> STSHCRFYENKYPEIDDIVMVNVQQIAEMGAYVKLLEYDNIEGMILLSELSRRRIRSIQKLIRVGKNDVA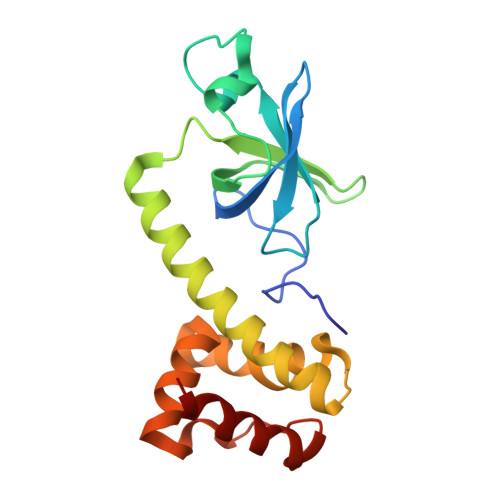VVLRVDKEKGYIDLSKRRVSSEDIIKCEEKYQKSKTVHSILRYCAEKFQIPLEELYKTIAWPLSRKFGHAYEAFKLSIIDETVWEGIEPPSKDVLDELKNYISKR>MKLSKDTTALLKNFATINSGIMLKSGQFIMTRAVNGTTYAEANISDVIDFDVAIYDLNGFLGILSLVNDDAEISQSEDGNIKIADARSTIFWPAADPSTVVAPNKPIPFPVASAVTEIKAEDLQQL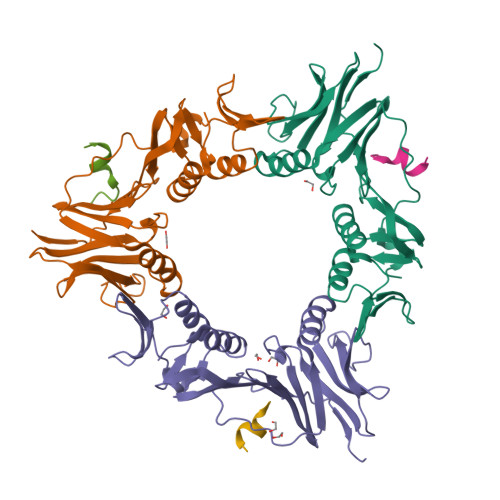LRVSRGLQIDTIAITVKEGKIVINGFNKVEDSALTRVKYSLTLGDYDGENTFNFIINMANMKMQPGNYKLLLWAKGKQGAAKFEGEHANYVVALEADSTHDFLEHHHHHH[3x];>KKEPEGLDFLFDA[3x]>[20x]PSLSKEAALVHEALVARGLETPLRPPVHEMDNETRKSLIAGHMTEIMQLLNLDLADDSLMET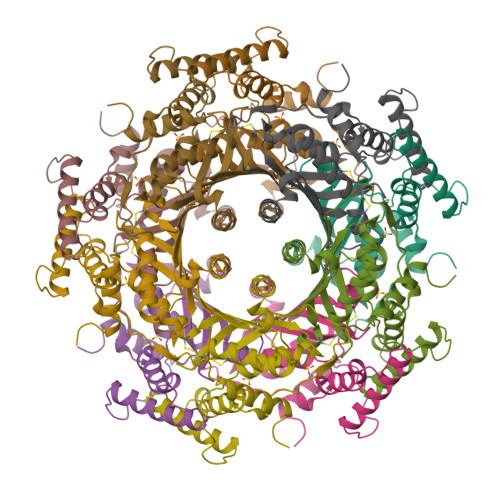PHRIAKMYVDEIFSGLDYANFPKITLIENKMKVDEMVTVRDITLTSTCEHHFVTIDGKATVAYIPKDSVIGLSKINRIVQFFAQRPQVQERLTQQILIALQTLLGTNNVAVSIDAVHYCVKARGIRDATSATTTTSLGGLFKSSQNTRHEFLRAVRHHN>GAMAHIHQLKAQGLPLPSNIPMIEINPTRVTLNMEFESQYYSLMTSDNGDHENVASIMAETNTLIQLPDRSVGGTTPDPFAQQVTITGYFGDVDRARMLMRRNCHFTVFMALSKMKMPLHELQAHVRQNPIQNVEMSFVDAPEKNGIVTTYLRITAREKNQHELIEAAKRLNEILFRESPAPENNFTLHFTLSTYYVDQVLGSSSTAQLMPVIERETTTIISYPCYNNRNETRGNIYEIKVVGNIDNVLKARRYIMDLLPISMCFNIKNTDMAEPSRVSDRNIHMIIDESGIILKMTPSVYEPADLLSGEVPLNCASLRSKEFNIKKLYTAYQKVLSKKFDF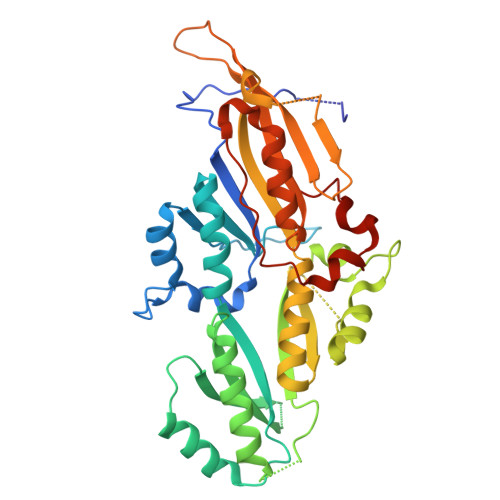IAPQPNDYDNSIWHHSLPANFLKNFNMPCRGELS[2x]>[2x]MSRPTIIINDLDAERIDILLEQPAYAGLPIADALN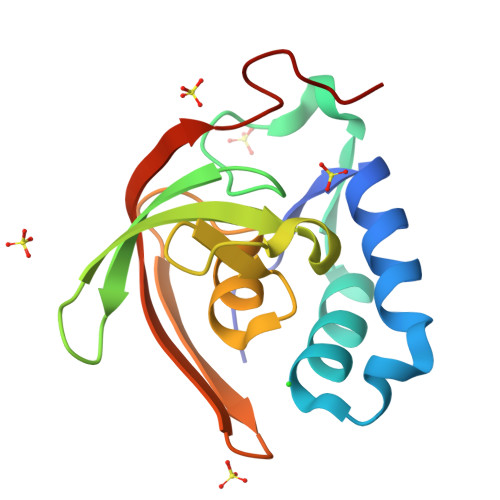AELDRAQMCSPEEMPHDVVTMNSRVKFRNLSDGEVRVRTLVYPAKMTDSNTQLSVMAPVGAALLGLRVGDSIHWELPGGVATHLEVLELEYQPEAAGDYLL> GSMKKERVITEFWDGKIIMVSPDDPKYALKKAEEVRELVDSELGFQQVSLRCPSQTRTYMFVSNEKKIVGCLIAEPIREAYRVLAEPPSLHSLHGEPLERHRAWRCSTEPEPAIC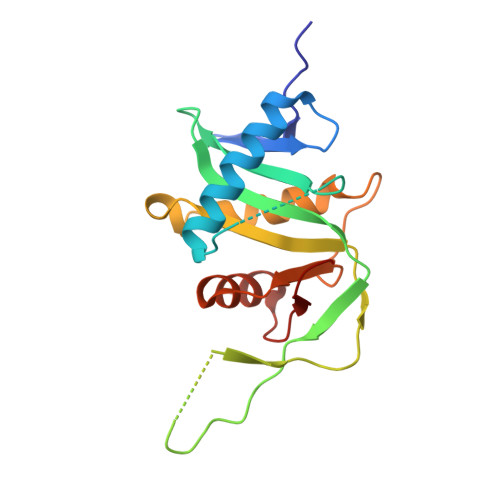GISRIWVFALMRRKAIASRMVDAVRSSFMYGSVLTTEEIAFSDPTPDGKLFASTYCKVPDFLVYNFVS>[5x]PSLEDLLFYTIAEGQEKIPVHKFITALKSTGLRTSDPRLKECMDMLRLTLQTTSDGVMLDKDLFKKCVQSNIVLLTQAFRRKLVIPDFMSFTSHIDELYESAKKQSGGKVA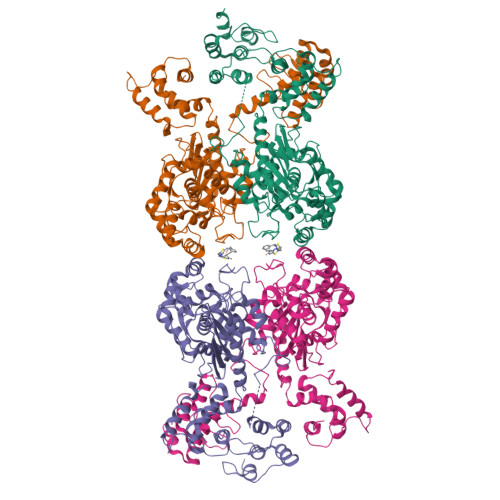DYIPQLAKFSPDLWGVSVCTVDGQRHSTGDTKVPFCLQSCVKPLKYAIAVNDLGTEYVHRYVGKEPSGLRFNKLFLNEDDKPHNPMVNAGAIVVTSLIKQGVNNAEKFDYVMQFLNKMAGNEYVGFSNATFQSERESGDRNFAIGYYLKEKKCFPEGTDMVGILDFYFQLCSIEVTCESASVMAATLANGGFCPITGERVLSPEAVRNTLSLMHSCGMYDFSGQFAFHVGLPAKSGVAGGILLVVPNVMGMMCWSPPLDKMGNSVKGIHFCHDLVSLCNFHNYDNLRHFAKKLDPRREGGDQRVKSVINLLFAAYTGDVSALRRFALSAMDMEQRDYDSRTALHVAAAEGHVEVVKFLLEACKVNPFPKDRWNNTPMDEALHFGHHDVFKILQEYQVQYTPQGDSDNGK>[2x]MIKSSFKAQPFLVRNTILCPNDKRSFTEYTQVIETVSKNKVFLEQLLLANPKLYDVMQKYNAGLLKKKRVKKLFESIYKYYKRSYLRSTPFGLFSETSIGVFSKSSQYKLMGKTTKGIRLDTQWLIRLVHKMEVDFSKKLS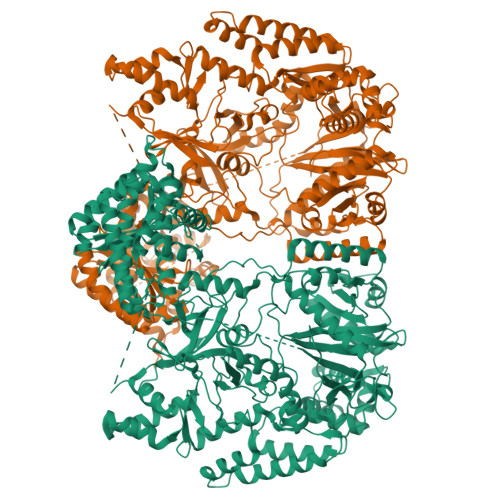FTRNNANYKFGDRVFQVYTINSSELEEVNIKYTNVYQIISEFCENDYQKYEDICETVTLCYGDEYRELSEQYLGSLIVNHYLISNLQKDLLSDFSWNTFLTKVEAIDEDKKYIIPLKKVQKFIQEYSEIEIGEGIEKLKEIYQEMSQILENDNYIQIDLISDSEINFDVKQKQQLEHLAEFLGNTTKSVRRTYLDDYKDKFIEKYGVDQEVQITELFDSTFGIGAPYNYNHPRNDFYESEPSTLYYSEEEREKYLSMYVEAVKNHNVINLDDLESHYQKMDLEKKSELQGLELFLNLAKEYEKDIFILGDIVGNNNLGGASGRFSALSPELTSYHRTIVDSVERENENKEITSCEIVFLPENIRHANVMHTSIMRRKVLPFFTSTSHNEVLLTNIYIGIDEKEKFYARDISTQEVLKFYITSMYNKTLFSNELRFLYEISLDDKFGNLPWELIYRDFDYIPRLVFDEIVISPAKWKIWGRDVNSKMTIRELIQSKEIPKEFYIVNGDNKVYLSQKNPLDMEILESAIKKSSKRKDFIELQEYFEDENIINKGEKGRVADVVVPFIRTRALGNEGRAFIREKRVSVERREKLPFNEWLYLKLYISINRQNEFLLSYLPDIQKIVANLGGNLFFLRYTDPKPHIRLRIKCSDLFLAYGSILEILKRSRKNRIMSTFDISIYDQEVERYGGFDTLELSEAIFCADSKIIPNLLTLIKDTNNDWKVDDVSILVNYLYLKCFFQNDNKKILNFLNLVSTKKVKENVNEKIEHYLKLLKVNNLGDQIFYDKNFKELKHAIKNLFLKMIAQDFELQKVYSIIDSIIHVHNNRLIGIERDKEKLIYYTLQRLFVSEEYMKTKDFNLDLVSVSK(2R)-3-{[(R)-hydroxy{[(1S,2R,3S,4S,5R,6R)-2,3,4,6-tetrahydroxy-5-(phosphonooxy)cyclohexyl]oxy}phosphoryl]oxy}propane-1,2-diyl 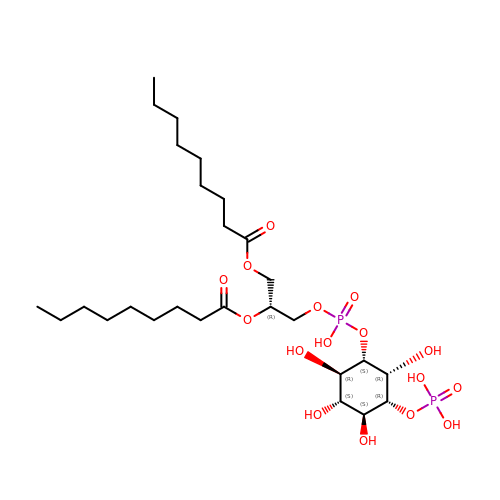dinonanoate | C27 H52 O16 P2 | IELCLCXLJSIZNX-ZAIPYKEWSA-N> GCGGGAGUGGCGAAAUUGGUAGACGCACCAGAUUUAGGUUCUGGCGCCGCAAGGUGUGCGAGUUCAAGUCUCG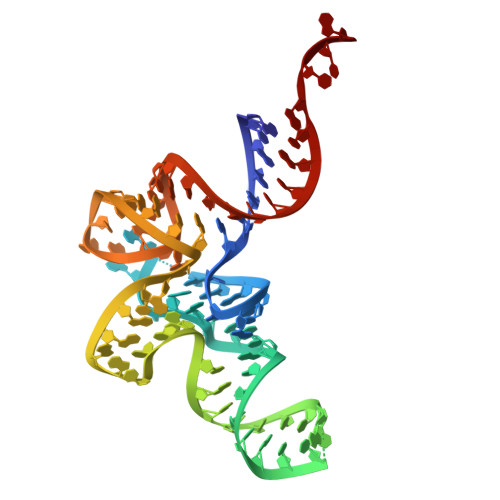CCUCCCGCACCA>MAALMTPGTGAPPAPGDFSGEGSQGLPDPSPEPKQLPELIRMKRDGGRLSEADIRGFVAAVVNGSAQGAQIGAMLMAIRLRGMDLEETSVLTQALAQSGQQLEWPEAWRQQLVDKHSTGGVGDKVSLVLAPALAACGCKVPMISGRGLGHTGGTLDKLESIPGFNVIQSPEQMQVLLDQAGCCIVGQSEQLVPADGILYAARDVTATVDSLPLITASILSKKLVEGLSALVVDVKFGGAAVFPNQEQARELAKTLVGVGASLGLRVAAALTAMDKPLGRCVGHALEVEEALLCMDGAGPPDLRDLVTTLGGALLWLSGHAGTQAQGAARVAAALDDGSALGRFERMLAAQGVDPGLARALCSGSPAERRQLLPRAREQEELLAPADGTVELVRALPLALVLHELGAGRSRAGEPLRLGVGAELLVDVGQRLRRGTPWLRVHRDGPALSGPQSRALQEALVLSDRAPFAAPSPFAELVLPPQQ[4x]

Human thymidine phosphorylase (hTP, EC 2.4.2.4), identified as the sole endothelial mitogenic and angiogenic factor, belongs to the pyrimidine nucleoside phosphorylase (PyNP) family. Thymidine phosphorylase, providing pyrimidine nucleotides for DNA repair and replication, has also been shown to have angiogenic activity in vivo. Here, we report the crystal structures of recombinant native hTP and in complex with 5-iodouracil (5IUR), a substrate with a Ki of 0.48 mM. The active site is located at the interface between the α- and the mixed α/β-domain.

The crystal structure of native hTP (at 3.0 Å) consists of two non-crystallographic dimers in the asymmetric unit. All four copies of hTP contain residues 34–479, residues 32 and 33 can be observed for chains A and B while only residue 33 can be observed for molecule C. At the C-terminal end, residue 480 was observed only in chain B. The crystal structure of hTP–5IUR complex (at 2.5 Å) consists of a dimer per asymmetric unit. No secondary structure differences were observed between native hTP, hTP–5IUR complex structure and the previously reported hTP structures. The crystal structure of unbound hTP provided some interesting findings. Alignment of the molecule A of the two structures (hTP and hTP–5IUR complex) indicates that they align well (including the flexible loop regions and the hinge region), with an rmsd of 0.57 Å over 445 Cα atoms. The ‘key hydrogen bond’ between His150 and Ala239 previously proposed to form the phosphate-binding site is present in both bound and unbound hTP structures. Hence, it is unlikely that only the binding of phosphate would trigger the formation of this key hydrogen bond as it is also observed in structures where a water molecule is present instead of a phosphate ion at the phosphate-binding site. Since no structure is available for the transition states of hTP, it is not possible to say conclusively whether any conformational change occurs during catalysis. It is evident that presence of substrate analogue is not required for the enzyme to acquire the ‘closed’ conformation. However, it is possible that the closed conformation observed for both bound and unbound hTP is favoured by crystal packing, while different ‘conformation/s’ of the enzyme may exist in solution.BAP29 and BAP31 are two homologous membrane proteins (∼50% sequence identity in humans) that reside in the endoplasmic reticulum (ER). They both consist of an N-terminal membrane-bound domain with three predicted transmembrane helices, and a C-terminal cytoplasmic region, which encompass ∼50% of the protein and is predicted to form a coiled coil, or more likely two coiled coils. BAP31 controls the fates of its bound clients, which may be either retained in the ER, progress through the secretory pathway or be extruded and subjected to ER-associated degradation. The structures presented here now show for the first time that the vDED domain adopts a dimeric coiled coil fold with no structural similarity to DED domains.

The structure of the vDED domain of BAP31 was determined in two different crystal forms; P21 at pH 8.0 and twinned P3221 at pH 4.2. The vDED domain forms an uninterrupted parallel coiled coil dimer in both structures. Almost all residues could be modeled in the P21 form (172–233), but not in the P3221 form (169–220). Apart from that, the two structures are however quite similar and exhibit a RMSD Cα value of 1.12 Å for 94 aligned residues. In the P21 form of BAP31 vDED, residues 204–233 of two dimers interact to form a tail-to-tail four-helical bundle across a crystal contact. This dimer-dimer interface covers an area of 2900 Å2 and is predicted by the PISA server to be stable in solution. For comparison, the radii of gyration (related to and numerically similar to the Stoke’s radius) of the dimer and potential tetramer of BAP31 vDED were estimated to be 29 and 39 Å respectively based on the P21 structure. We therefore conclude that BAP31 vDED elute as a dimer on the gel filtration column at pH 7.0. We therefore conclude that the observed tetramerization interface is unlikely to be physiologically relevant.

>SMLDVGNAEVKLEEENRSLKADLQKLKDELASTKQKLEKAENQVLAMRKQSEGLTKEYDRLLEEHAKL[4x]> MDDCSGKTDAWTSIKGPKTGGYWLKQTTKTGENECTYVKGTDFKENTKTATYTYGYKDASGKLTKTTGTAMAKGSDIVVGSDTSTVIYTDGKTCDVVKHGGHTELWVH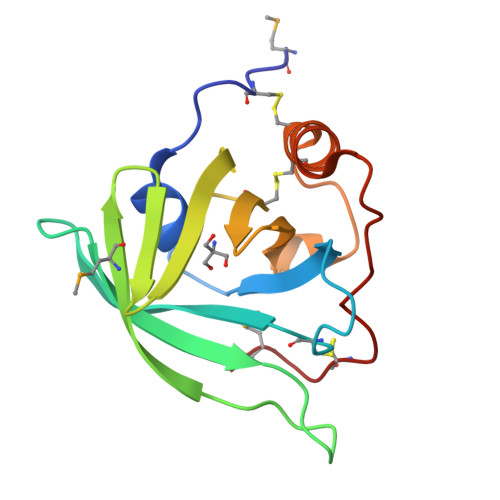SSKTSGGYNNCCDKKFTETRGSTPANEVYKKCPGMP>CGCGGCGUUGCGUCCGAAAGUCUAAACAGACACGGCCGCUUAAAAACAAAAGGAGA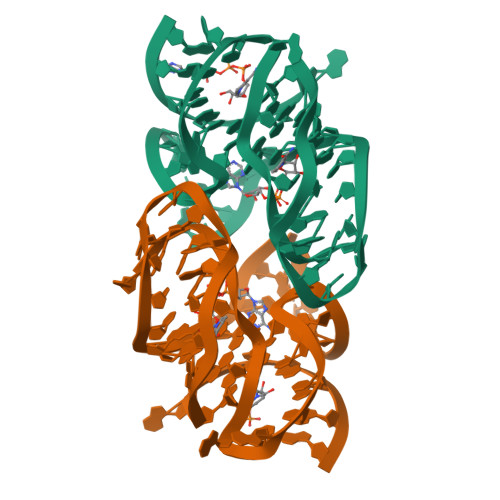[2x]> AVSFIGSTENDVGPSQGSYSSTHAMDNLPFVYNTGHNIGYQNANVWRISGGFCVGLDGKVDLPVVGSLDGQSIYGLTEEVGLLIWMGDTNYSRGTAMSGNSWENVFSGWCVGNYVSTQG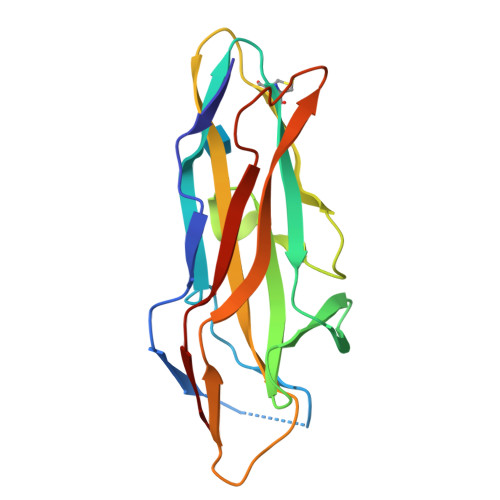LSVHVRPVILKRNSSAQYSVQKTSIGSIRMRPYNGSSAGSVQTTVNFSLNPFTLNDT> MLPKRRRARVGSPSGDAASSTPPSTRFPGVAIYLVEPRMGRSRRAFLTGLARSKGFRVLDACSSEATHVVMEETSAEEAVSWQERRMAAAPPGCTPPALLDISWLTESLGAGQPVPVECRHRLEVAGPRKGPLSPAWMPAYACQRPTPLTHHNTGLSEALEILAEAAGFEGSEGRLLTFCRAASVLKALPSPVTTLSQLQGLPHFGEHSSRVVQELLEHGVCEEVERVRRS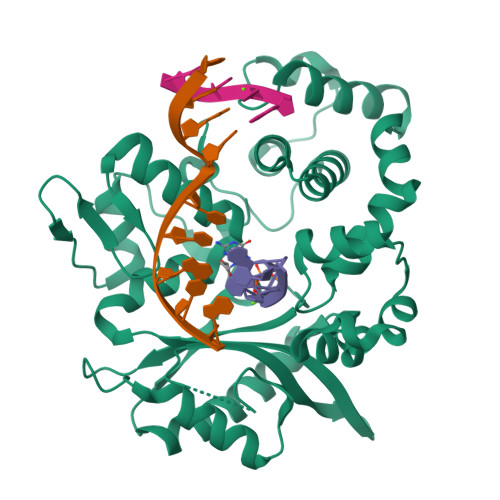ERYQTMKLFTQIFGVGVKTADRWYREGLRTLDDLREQPQKLTQQQKAGLQHHQDLSTPVLRSDVDALQQVVEEAVGQALPGATVTLTGGFRRGKLQGHDVDFLITHPKEGQEAGLLPRVMCRLQDQGLILYHQHQHSCCESPTRLAQQSHMDAFERSFCIFRLPQPGSWKAVRVDLVVAPVSQFPFALLGWTGSKLFARELRRFSRKEKGLWLNSHGLFDPEQKTFFQAASEEDIFRHLGLEYLPPEQRNA> LPSYVDWRSAGAVVDIKSQGECGGCWAFSAIATVEGINKITSGSLISLSEQELIDCGRTQNTRGCDGGYITDG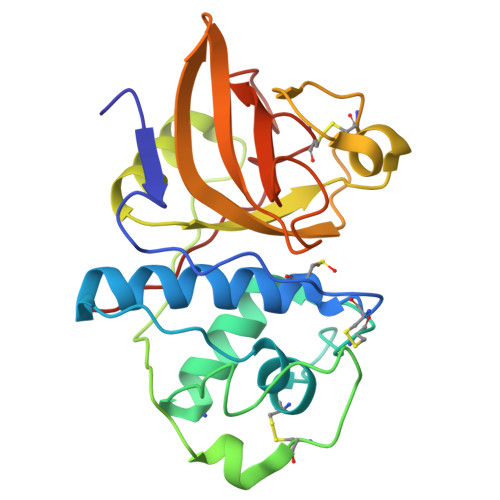FQFIINDGGINTEENYPYTAQDGDCDVALQDQKYVTIDTYENVPYNNEWALQTAVTYQPVSVALDAAGDAFKQYASGIFTGPCGTAVDHAIVIVGYGTEGGVDYWIVKNSWDTTWGEEGYMRILRNVGGAGTCGIATMPSYPVKYNN>[2x]GAMGDFSFIKALQTAQQNFVVTDPSLPDNPIVYASQGFLNLTGYSLDQILGRNCRFLQGPETDPKAVERIRKAIEQGNDMSVCLLNYRVDGTTFWNQFFIAALRDAGGNVTNFVGVQCKVSDQYAATVTKQQEEEEEAAANDDED

Aureos typically consist of an N-terminal domain with unknown function, a basic region leucine zipper (bZIP) DNA-binding domain, and a C-terminal light-oxygen-voltage (LOV) sensing domain. LOV domains are a subgroup of the Per-Arnt-Sim (PAS) superfamily that sense blue light using a noncovalently bound flavin cofactor. Photon absorption of the flavin results in formation of a flavin-C4(a)-cysteinyl adduct with a conserved cysteine residue, which initiates a cascade of structural rearrangements within the LOV core that are propagated to the domain boundaries. Here, we present crystal structures of a fully light-adapted LOV dimer as well as of a dark state LOV monomer of PtAu1a.

The dark state structure revealed a LOV monomer that adopts a typical PAS fold consisting of a five-stranded antiparallel β-sheet flanked by several helices. The LOV core forms the chromophore binding pocket and closely resembles the structure of VfAu1 LOV (root-mean-square deviation (r.m.s.d) between 0.42 and 0.58 Å for 101 Cα atoms and molecules A and B PtAu1a and A,B,C,D,E,F for VfAu1a). The LOV core is flanked at the N- and C-termini by prominent α-helical extensions denoted A´α and Jα, respectively. As observed for VfAu1 LOV, the C-terminal Jα helix partially folds back onto the surface of the β-sheet and interacts with the LOV core via hydrogen bonds between the conserved residue Gln365 and the carbonyl and amine group of Cys316 as well as the side chains of Tyr357 and Gln330. A´α forms an amphipathic three-turn helix and interacts with the LOV core through a highly conserved 4 amino acid linker with Ala248, Glu249, Glu250 and Gln251 in the hinge region. In addition to Jα, A´α also folds back across the surface of the β-sheet and covers a large hydrophobic patch. The chromophore binding pocket is mainly formed by hydrophobic residues that stabilize the FMN chromophore together with Gln350, Gln291, Asn319, Asn329, which form hydrogen bonds with the heteroatoms of the isoalloxazine ring. FMN is additionally stabilized by Arg304 and Arg288, which interact with the phosphate group of the ribityl chain. In the dark, A'α covers the hydrophobic dimerization site of the LOV β-sheet that becomes exposed upon illumination and thus enables LOV dimerization. Crystallization of PtAu1aLOV was performed at 20°C. Dark state crystals were grown in sitting-drop geometry with unreconstituted PtAu1aLOV protein (chromophore occupancy ~55%, protein buffer: 20 mM Tris pH 8.0, 100 mM NaCl, 10% (w/v) glycerol) using a protein concentration of 16 mg ml–1 and 40% (v/v) ethylene glycol and 0.1 M sodium acetate pH 4.5 as reservoir solution.>[4x]GSHMPGFYEIVIKVPSDLDGHLPGISDSFVNWVAEKEWELPPDSDMDLNLIEQAPLTVAEKLQRDFLTEWRR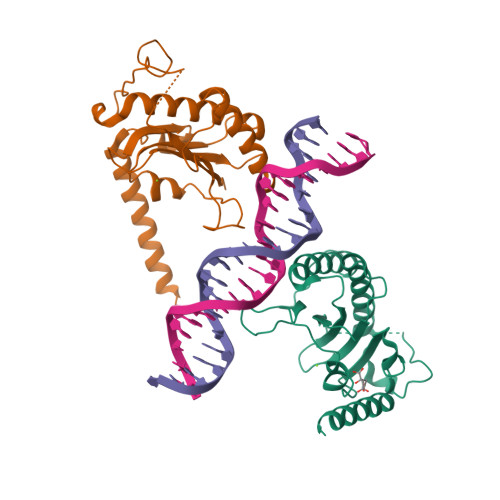VSKAPEALFFVQFEKGESYFHMHVLVETTGVKSMVLGRFLSQIREKLIQRIYRGIEPTLPNWFAVTKTRNGAGGGNKVVDESYIPNFLLPKTQPELQWAWTNMEQYLSACLNLTERKRLVAQHLTHVSQTQEQNKENQNPN> GANRTLIVTTILEEPYVMYRKSDKPLYGNDRFEGYCLDLLKELSNILGFLYDVKLVPDGKYGAQNDKGEWNGMVKELIDHRADLAVAPLTITYVREKVIDFSKPFMTLGISILYRKGTPIDSADDLAKQTKIEYGAVRDGSTMTFFKKSKISTYEKMWAFMSSRQQSALVKNSDEGIQRVLTTDYALLMES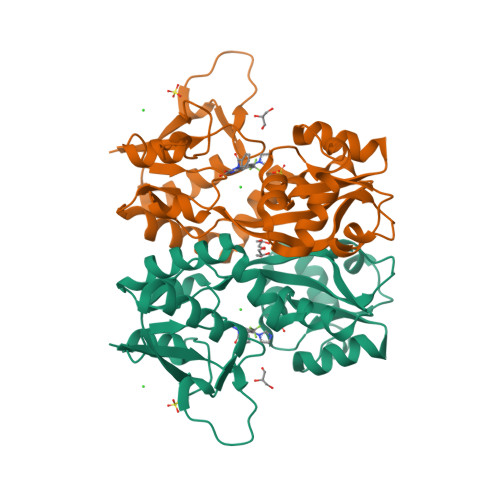TSIEYVTQRNCNLTQIGGLIDSKGYGVGTPIGSPYRDKITIAILQLQEEGKLHMMKEKWWRGNGCP dodecyl 1H-benzimidazole-5-carboxylate | C20 H30 N2 O2 | 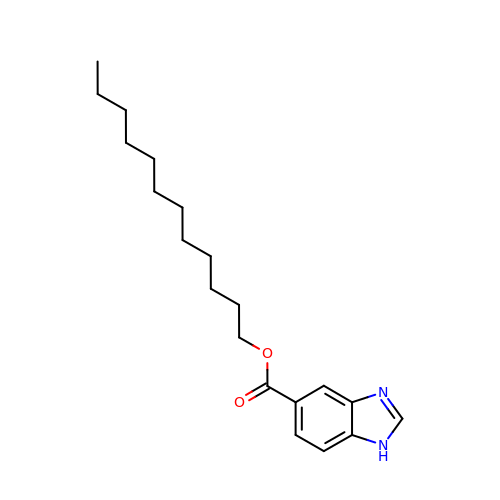VXKKXAFRWVJMCS-UHFFFAOYSA-N> MAHHHHHHHHHANVVVCIKQVPDTTNVRIDRKTNNLVREGVPSIINPDDERALELASQL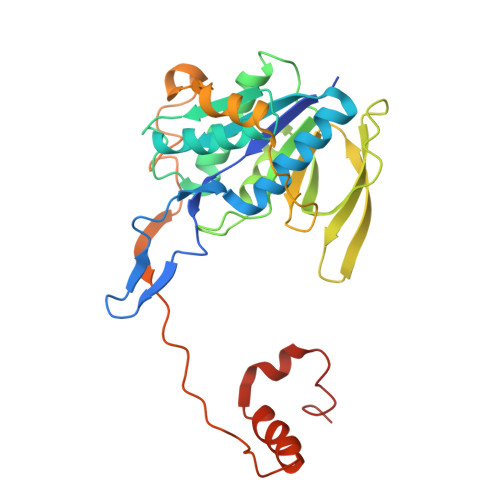KEKFGATVYVITMGPPQAKEALKDAIAFGLDEAVHLSDRTFAGADTLATTYTLYWGIKKIEERIGKIDLILTGKQAVDGDTGQVGPGLATRFGYALGAYVVRIEEIDPEKKEMVIVRRLDQGFEKIRLKLPAVLTITDELNKPRYADLPNLIRAIRYEPIVWTHKDLGLDPKKCGFFGSPTRVVSTNIPPARKGGDIISKNEDPEVAAEKLIEALKKFEAVRLVEALKPVLEGEKDE>MAANMYRVGDYVYFENSSSNPYLIRRIEELNKTANGNVEAKVVCFYRRRDISSTLIALADKHATLSVCYKAGPGADNGEEGEIEEEMENPEMVDLPEKLKHQLRHRELFLSRQLESLPATHIRGKCSVTLLNETESLKSYLEREDFFFYSLVYDPQQKTLLADKGEIRVGNRYQADITDLLKEGEEDGRDQSRLETQVWEAHNPLTDKQIDQFLVVARSVGTFARALDCSSSVRQPSLHMSAAAASRDITLFHAMDTLHKNIYDISKAISALVPQGGPVLCRDEMEEWSASEANLFEEALEKYGKDFTDIQQDFLPWKSLTSIIEYYYMWKTTDRYVQQKRLKAAEAESKLKQVYIPNYNKPNPNQISVNNVKAGVVNGTGAPGQSPGAGRACESCYTTQSYQWYSWGPPNMQCRLCASCWTYWKKYGGLKMPTRLDGERPGPNRSNMSPHGLPARSSGSPKFAMKTRQAFYLHTTKLTRIARRLCREILRPWHAARHPYLPINSAAIKAECTARLPEASQSPLVLKQAVRKPLEAVLRYLETHPRPPKPDPVKSVSSVLSSLTPAKVAPVINNGSPTILGKRSYEQHNGVDGNMKKRLLMPSRGLANHGQARHMGPSRNLLLNGKSYPTKVRLIRGGSLPPVKRRRMNWIDAPDDVFYMATEETRKIRKLLSSSETKRAARRPYKPIALRQSQALPPRPPPPAPVNDEPIVIED[2x];>MAQTQGTRRKVCYYYDGDVGNYYYGQGHPMKPHRIRMTHNLLLNYGLYRKMEIYRPHKANAEEMTKYHSDDYIKFLRSIRPDNMSEYSKQMQRFNVGEDCPVFDGLFEFCQLSTGGSVASAVKLNKQQTDIAVNWAGGLHHAKKSEASGFCYVNDIVLAILELLKYHQRVLYIDIDIHHGDGVEEAFYTTDRVMTVSFHKYGEYFPGTGDLRDIGAGKGKYYAVNYPLRDGIDDESYEAIFKPVMSKVMEMFQPSAVVLQCGSDSLSGDRLGCFNLTIKGHAKCVEFVKSFNLPMLMLGGGGYTIRNVARCWTYETAVALDTEIPNELPYNDYFEYFGPDFKLHISPSNMTNQNTNEYLEKIKQRLFENLRMLPHAPGVQMQAIPEDAIPEESGDEDEDDPDKRISICSSDKRIACEEEFSDSEEEGEGGRKNSSNFKKAKRVKTEDEKEKDPEEKKEVTEEEKTKEEKPEAKGVKEEVKLA[2x];> MRAHPGGGRCCPEQEEGESAAGGSGAGGDSAIEQGGQGSALAPSPVSGVRREGARGGGRGRGRWKQAGRGGGVCGRGRGRGRGRGRGRGRGRGRGRPPSGGSGLGGDGGGCGGGGSGGGGAPRREPVPFPSGSAGPGPRGPRATESGKRMDCPALPPGWKKEEVIRKSGLSAGKSDVYYFSPSGKKFRSKPQLARYLGNTVDLSSFDFRTGKMMPSKLQKNKQRLRNDPLNQNKGKPDLNTTLPIRQTASIFKQPVTKVTNHPSNKVKSDPQRMNEQPRQLFWEKRLQGLSASDVTEQIIKTMELPKGLQGVGPGSNDETLLSAVASALHTSSAPITGQVSAAVEKNPAVWLNTSQPLCKAFIVTDEDIRKQEERVQQVRKKLEEALMADILSRAADTEEMDIEMDSGDEA

The Nucleosome Remodelling and Deacetylase (NuRD) complex is a multi-protein chromatin modifying machine that plays an essential role in cell lineage commitment and DNA damage repair. The complex controls expression of genes through two distinct activities: removal of acetyl groups from chromatin through the action of a histone deacetylase enzyme and remodelling of nucleosomes through an ATP-dependent helicase. The deacetylase module from the NuRD complex contains three protein domains that control the recruitment of chromatin to the deacetylase enzyme, HDAC1/2. Using biochemical approaches and cryo-electron microscopy, we have determined how three chromatin-binding domains (MTA1-BAH, MBD2/3 and RBBP4/7) are assembled in relation to the core complex so as to facilitate interaction of the complex with the genome.

To visualise how MBD2 interacts with the HDAC1:MTA1 dimer we used cryo-electron microscopy to determine the structure of MBD2 bound to the MTA1(ELM2-SANT):HDAC1 complex. A map was calculated using 70 561 particles to a resolution of 6.1 Å. The dimeric nature of the complex was immediately apparent in the raw micrographs with front-on particles resembling ‘bowties’ (i.e. two HDACs flanking the MTA1 dimer interface). On fitting the HDAC1:MTA1 dimer structure into the map, it was apparent that the complex was asymmetric with additional density appearing on one but not both of the MTA1-SANT domains. Having placed the two crystal structures into the map, the remaining unaccounted-for density was extracted and examined. Particularly interesting was density from the intrinsically disordered domain (IDR) of MBD2, and the CC domain, which appears to wrap around both sides of the dimerisation interface. On inspection of the MBD2 sequence we identified a short hydrophobic motif (I/VTxQI/V) that is repeated twice in MBD2 with a linker of 36 amino-acids. Binding of the two motifs across the MTA1 dimer interface would explain why one bound MBD2 would occlude binding of a second MBD2. The 3D map was high enough resolution to model a single MBD domain (MBD2 residues 145–220) in close proximity to one of the MTA1-SANT domains. MBD2 appears to wrap around the dimerisation interface of MTA1, binding to both front and back surfaces, possibly through a repeated motif.>PPGTVDKKMVEKCWKLMDKVVRLCQNPKLALKNSPPYILDLLPDTYQHLRTILSRYEGKMETLGENEYFRVFMENLMKKTKQTISLFKEGKERMYEENSQPRRNLTKLSLIFSHMLAELKGIFPSGLFQGDTFRITKADAAEFWRKAFGEKTIVPWKSFRQALHEVHPISSGLEAMALKSTIDLTCNDYISVFEFDIFTRLFQPWSSLLRNWNSLAVTHPGYMAFLTYDEVKARLQKFIHKPGSYIFRLSCTRLGQWAIGYVTADGNILQTIPHNKPLFQALIDGFREGFYL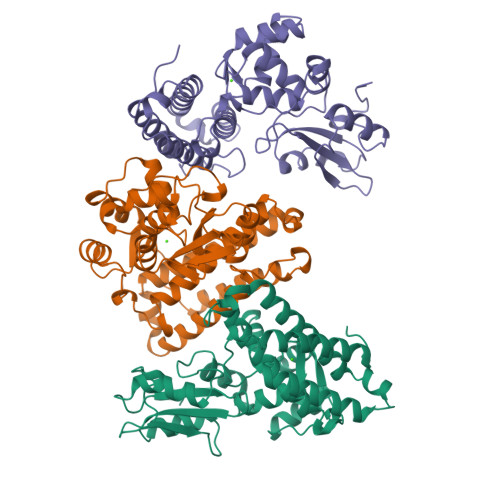FPDGRNQNPDLT[3x]> MSRNPSNSDAAHAFWSTQPVPQTEDETEKIVFAGPMDEPKTVADIPEEPYPIASTFEWWTPNMEAADDIHAIYELLRDNYVEDDDSMFRFNYSEEFLQWALCPPSYIPDWHVAVRRKADKKLLAFIAGVPVTLRMGTPKYMKVKAQEKGQEEEAAKYDAPRHICEINFLCVHKQLREKRLAPILIKEVTRRVNRTNVWQAVYTAGVLLPTPYASGQYFHRSLNPEKLVEIRFSGIPAQYQKFQNPMAMLKRNYQLPNAPKNSGLREMKPSDVPQVRRILMNYLDNFDVGPVFSDAEISHYLLPRDGVVFTYVVENDKKVTDFFSFYRIPSTVIGNSNYNILNAAYVHYYAATSMPLHQLILDLLIVAHSRGFDVCNMVEILDNRSFVEQLKFGAGDGHLRYYFYNWAYPKIKPSQVALVML

NMT is ubiquitous in eukaryotic cells in which it catalyses the co-translational addition of the C14:0 fatty acid, myristate, via an amide bond, to the N-terminal glycine residue of a subset of proteins. N-Myristoylation by NMT proceeds via an ordered Bi–Bi reaction mechanism; binding of myristoyl-CoA opens up a second pocket for docking of the substrate protein. The myristate group is then transferred to the N-terminal glycine of the substrate in a nucleophilic addition–elimination reaction, followed by stepwise release of first the free CoA and then the N-myristoylated protein. Here, we extend our studies on NMT to Leishmania donovani (LdNMT), the principal causative agent of the most serious form of leishmaniasis, and demonstrate that the L. donovani NMT gene is also likely to be essential for viability in extracellular parasites.

LdNMT was co-crystallised with NHM, a non-hydrolysable analogue of myristoyl-CoA with a methylene group intervening between the sulfur and the carbonyl carbon in what would otherwise be the thioester linkage in myristoyl-CoA. The refined coordinates have good agreement with the X-ray data extending to 1.42 Å resolution, with Rcryst and Rfree values of 14.6% and 19.1%, respectively. There is a single LdNMT molecule in the asymmetric unit and the chain is well defined in the electron density maps, with the exception of residues 1–10 at the amino terminus and residues 83–85 and 334–339, which are not defined by the maps and assumed to be disordered. All 64 heavy atoms of the NHM are clearly defined in the electron density maps with this ligand residing in one side of a prominent groove running across the molecule. The fatty acyl-CoA binds to the N-terminal lobe in a site that is formed by the eCf elements that encircle the cofactor, with the A′ 310 helix and the Ab loop forming lateral interactions. In its bound conformation, 1070 Å2 or 88% of the cofactor's solvent-accessible surface area of 1215 Å2 is buried by interaction with the protein. The carbonyl group of the pentadecyl moiety is directed into the protein interior to form hydrogen bonds with the main-chain amide groups of Phe168 and Leu169, these groups forming the oxyanion hole. It runs into a deep hydrophobic pocket lined by residues Trp15, Ile166, Leu169, Ile185, Val192, Trp198, Gln199, Ala200, Tyr202, Leu208, and Tyr404. The most striking distinguishing feature of LdNMT is the additional pair of α-helices C′ and C″. These structural elements correspond to a prominent ∼ 20-residue insertion at residue 140 in the sequence of the Leishmania NMTs.>MHHHHHHTSKIEQPRWASKDSAAGAASTPDEKIVLEFMDALTSNDAAKLIEYFAEDTMYQNMPLPPAYGRDAVEQTLAGFFTVFSIDAVETFHIGSSNGLVYTERVDVVRALPTGKSYNVSVLGVFQLTEGKITGWRDYFD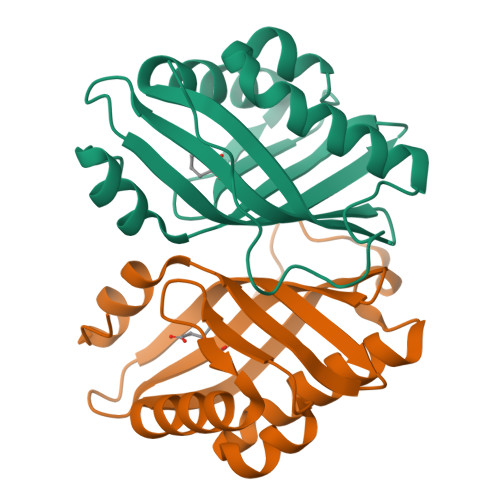LREVEEAVDLPVRG[4x]> MSFPLIFERSRKGRRGLKLVKAVPKAEDLIPKEHLREVPPRLPEVDELTLVRHYTGLSRRQVGVDTTFYPLGSCTMKYNPKLHEEAARLFADLHPYQDPRTAQGALRLMWELGEYLKALTGMDAITLEPAAGAHGELTGILIIRAYHE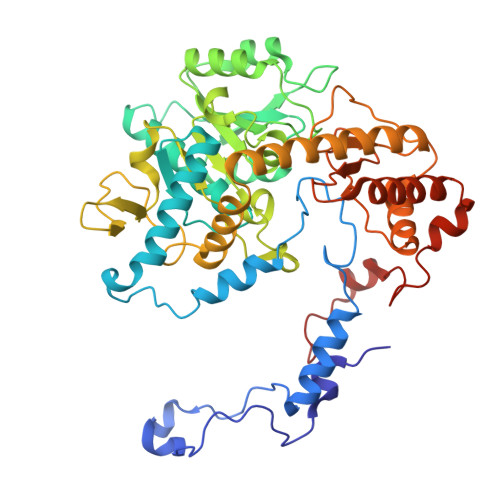DRGEGRTRRVVLVPDSAHGSNPATASMAGYQVREIPSGPEGEVDLEALKRELGPHVAALMLTNPNTLGLFERRILEISRLCKEAGVQLYYDGANLNAIMGWARPGDMGFDVVHLNLHKTFTVPHGGGGPGSGPVGVKAHLAPYLPVPLVERGEEGFYLDFDRPKSIGRVRSFYGNFLALVRAWAYIRTLGLEGLKKAAALAVLNARYLKELLKEKGYRVPYDGPSMHEFVAQPPEGFRALDLAKGLLELGFHPPTVYFPLIVKEALMVEPTETEAKETLEAFAEAMGALLKKPKEWLENAPYSTPVRRLDELRANKHPKLTYFDEG>MNGPIIMTREERMKIVHEIKERILDKYGDDVKAIGVYGSLGRQTDGPYSDIEMMCVMSTEEAEFSHEWTTGEWKVEVNFYSEEILLDYASQVESDWPLTHGQFFSILPIYDSGGYLEKVYQTAKSVEAQKFHDAICALIVEELFEYAGKWRNIRVQGPTTFLPSLTVQVAMAGAMLIGLH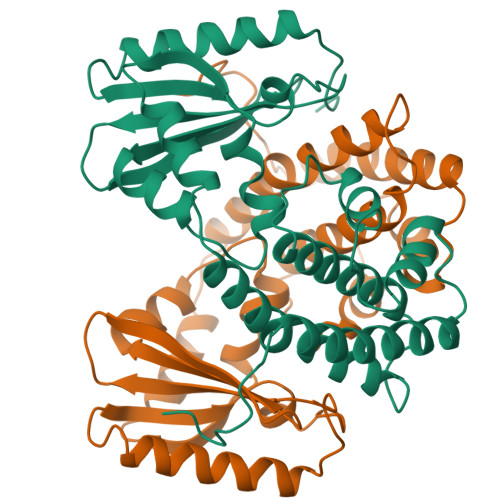HRICYTTSASVLTEAVKQSDLPSGYDHLCQFVMSGQLSDSEKLLESLENFWNGIQEWTERHGYIVDVSKRIPF[2x]>ADPALADVCRTKLPSQAQDTLALIAKNGPYPYNRDGVVFENRESRLPKKGNGYYHEFTVVTPGSNDRGTRRVVTGGYGEQYWSPDHYATFQE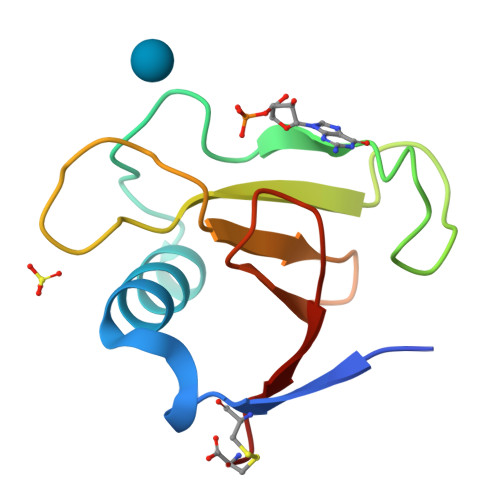IDPRC[4x]HEXYLPHOSPHONIC ACID (R)-2-METHYL-3-PHENYLPROPYL ESTER | C16 H27 O3 P | 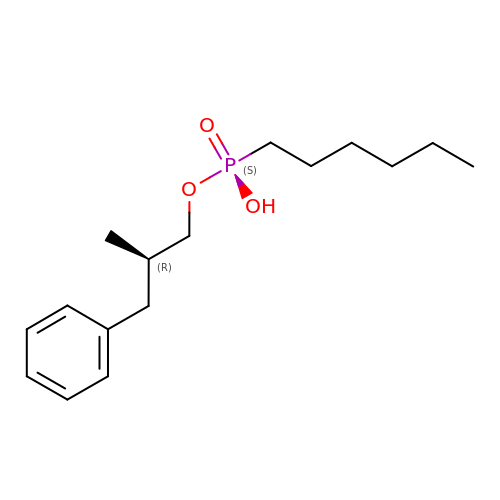MMTDYBZZRYOMFD-OAHLLOKOSA-N> GVALGATRVIYPAGQKQEQLAVTNNDENSTYLIQSWVENADGVKDGRFIVTPPLFAMKGKKENTLRILDATNNQLPQDRESLFWMNVKAIPSMDKSKLTENTLQLAIISRIKLYYRPAKLALPPDQAAEKLRFRRSANSLTLINPTPYYLTVTELNAGTRVLENALVPPMGESTVKLPSDAGSNITYRTINDYGALTPKMTGVME;> DLYFNPRFLADDPQAVADLSRFENGQELPPGTYRVDIYLNNGYMATRDVTFNTGDSEQGIVPCLTRAQLASMGLNTASVAGMNLLADDACVPLTTMVQDATAHLDVGQQRLNLTIPQAFMSNRAR;> TGGCDVSARDVTVTLPDYPGSVPIPLTVYCAKSQNLGYYLSGTTADAGNSIFTNTASFSPAQGVGVQLTRNGTIIPANNTVSLGAVGTSAVSLGLTANYARTGGQVTAGNV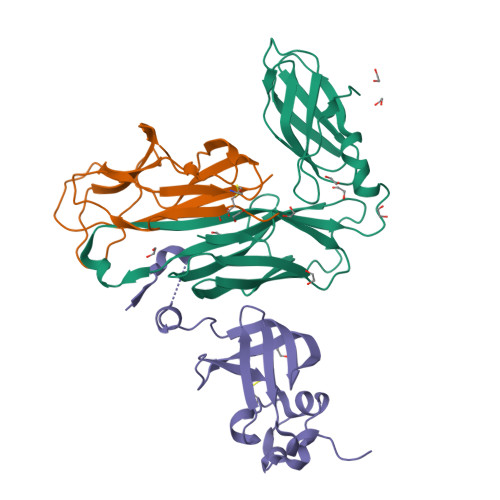QSIIGVTFVYQ>[4x]MEINGVEIEDTYAEAFPIKIARVLITAATKRWALVAATEATGFATSVIMCPAEAGIERLASPSETPDGRPGVYVQICTFKYEALEEQLLERIGQCVLTAPTTAVFNGLPEAEKQDNVGFKLKFFADGMESETQIAGRKVYKVPIMEGDFLA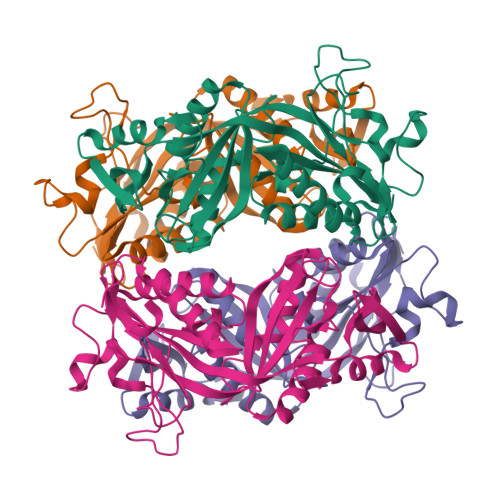EENIGAIAGIAGGNFFIFGDSQMTALTAAEAAVDTIAELEGTITPFPGGIVASGSKSGANKYKFLKATANERFCPSIKDKIENTEIPADVNAVYEIVINGLDEESIKAAMKAGIKAAVTVPGVKKISAGNYGGKLGKYQFKLHELF>MASPNPLAFEAATAAHEVAASYVTEHKPRKNDNINFANFNQDFSCVSVGYSNGYKIYNCEPFGQCYSKSDGSIGIVEMLFSSSLLAIVGMGEQHSLSPRRLKIINTKRQTTICELTFPGAILAVKLNRERLVVLLEETIYIYDINNMRLLHTIETPSNPNGLIALSPSSENNYLAYPSPQKLAPNPQTEVTLHSNPQTVRNGDVIIFDAKTLQPTSVIEAHRTSLAAIALSKDGLLLATASDKGTIIRVFSVATGIKLYQFRRGTYPTKIYSLAFSPDNRFVIASSATETVHIFRLGEEEAANTIKSANKKARLTKAQVPNPLETSPDIYPHNQHTSSDEDEELNEDEEDLDGDEDEDLEDDAHVPVSLQRGRSSSSTGSFHSSESMTDKLKEPLVDNSRKSVARMLRRTSQSLGRKAAEKMGTYLPPKFSSILEPNRHFASLKVPASKETKTVVG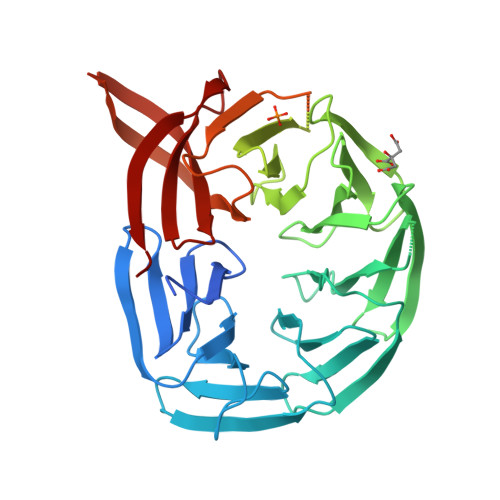VGSKIWDDLIPSVYLKDDANSITETSEDLVNKKLVHIMVITSEGFFYKFGLDPERGGDCVLLHQQSLFG[2x]> MDTWTVLLILQASLVLPGAVGTRTNTRTTPTPILRFVAVGDWGGVPNAPFHTAREMANAKAIATTVKTLGADFILSLGDNFYFTGVHDAKDKRFQETFEDVFSDPSLRNVPWHVLAGNHDHLGNVSAQIAYSKISKRWNFPSPYYRLRFKIPRSNVSVAIFMLDTVTLCGNSDDFVSQQPERPRNLALARTQLAWIKKQLAAAKEDYVLVAGHYPVWSIAEHGPTHCLVKQLLPLLTTHKVTAYLCGHDHNLQYLQDENGLGFVLSGAGNFMDPSKKHLRKVPNGYLRF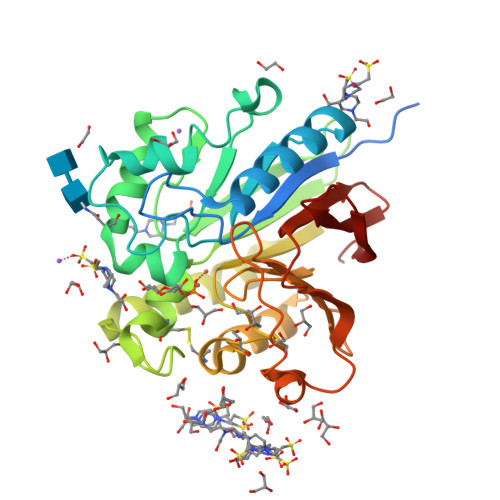HFGAENSLGGFAYVEITPKEMSVTYIEASGKSLFKTKLPRRA> MVPISPIETVPVKLKPGMDGPKVKQWPLTEEKIKALVEICTEMEKEGKISKIGPENPYNTPVFAIKKKDSTKWRKLVDFRELNKRTQDFWEVQLGIPHPAGLKKKKSVTVLDVGDAYFSVPLDEDFRKYTAFTIPSINNETPGIRYQYNVLPQGWKGSPAISQSSMTKILEPFKKQNPDIVIYQYMDDLYVGSDLEIGQHRTKIEELRQHLLRWGLTTPDKKHQKEPPFLWMGYELHPDKWTVQPIVLPEKDSWTVNDIQKLVGKLNWASQIYPGIKVRQLSKLLRGTKALTEVIPLTEEAELELAENREILKEPVHGVYYDPSKDLIAEIQKQGQGQWTYQIYQEPFKNLKTGKYARMRGAHTNDVKQLTEAVQKITTESIVIWGKTPKFKLPIQKETWETWWTEYWQATWIPEWEFVNTPPLVKLWYQLEKEPIVGAETFYVDGAANRETKLGKAGYVTNKGRQKVVPLTNTTNQKTELQAIYLALQDSGLEVNIVTDSQYALGIIQAQPDKSESELVNQIIEQLIKKEKVYLAWVPAHKGIGGNEQVDKLVSAG;> PISPIETVPVKLKPGMDGPKVKQWPLTEEKIKALVEICTEMEKEGKISKIGPENPYNTPVFAIKKKDSTKWRKLVDFRELNKRTQDFWEVQLGIPHPAGLKKKKSVTVLDVGDAYFSVPLDEDFRKYTAFTIPSINNETPGIRYQYNVLPQGWKGSPAIFQSSMTKILEPFKKQNPDIVIYQYMDDLYVGSDLEIGQHRTKIEELRQHLLRWGLTTPDKKHQKEPPFLWMGYELHP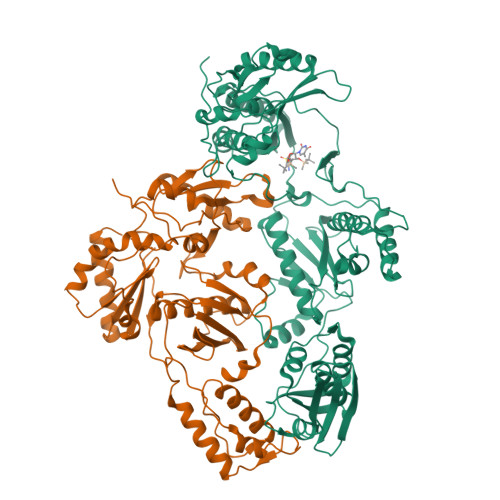DKWTVQPIVLPEKDSWTVNDIQKLVGKLNWASQIYPGIKVRQLSKLLRGTKALTEVIPLTEEAELELAENREILKEPVHGVYYDPSKDLIAEIQKQGQGQWTYQIYQEPFKNLKTGKYARMRGAHTNDVKQLTEAVQKITTESIVIWGKTPKFKLPIQKETWETWWTEYWQATWIPEWEFVNTPPLVKLWYQ>[2x]GPLGSHMNINRQLPVSGSERLLTPDVGVSRQACSERHYSTGQDRHDFYRFAARLHVDAQCFGLSIDDLMDKFSDKHFRAEHPEYRDVYPEECSAIYMHTAQDYSSHLVRGEIGTPLYREVNNYLRLQHENSGREAEIDNHDEKLSPHIKMLSSALNRLMDVAAFRGTVYRGIRGDLD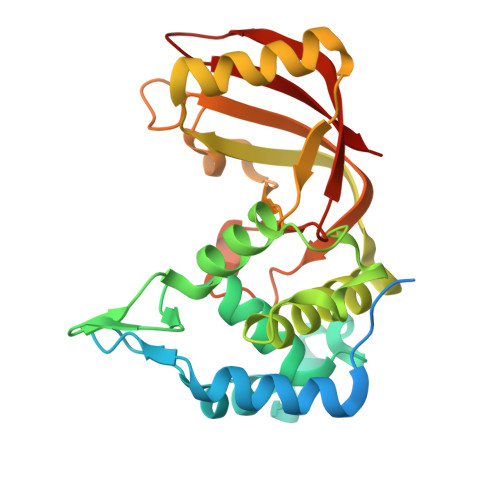TIARLYHLFDTGGRYVEPAFMSTTRIKDSAQVFEPGTPNNIAFQISLKRGADISGSSQAPSEEEIMLPMMSEFVIEHASALSEGKHLFVLSQI>MRGSHHHHHHGSMSNVLIFNVGSSSLTYKVFCSDNIVCSGKSNRVNVTGTEKPFIEHHLNGQIIKIETPILNHPQAAKLIIQFLKENHISIAFVGHRFVHGGSYFKKSAVIDEVVLKELKECLPLAPIHNPSSFGVIEISMKELPTTRQYVAIDTAFHSTISQAERTYAIPQPYQSQYLKFGFHGLSYEYVINSLKN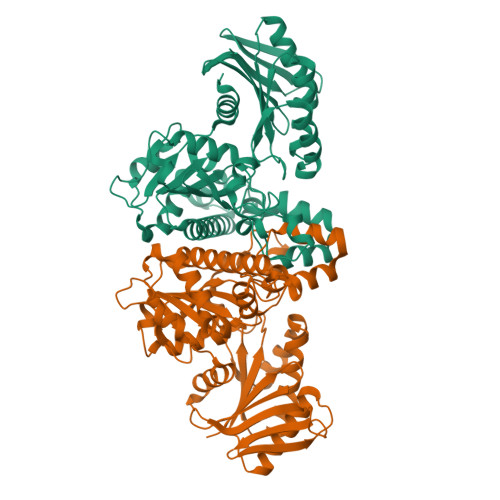VIDVSHSKIIACHLGTGGSSCCGIVNGKSFDTSMGNSTLAGLVMSTRCGDIDPTIPIDMIQQVGIEKVVDILNKKSGLLGVSELSSDMRDILHEIETRGPKAKTCQLAFDVYIKQLAKTIGGLMVEIGGLDLLVFTDQMGLEVWQVRKAICDKMKFLGIELDDSLNEKSMGKKIEFLTMPSSKVQVCVAPNDEELVILQKGKELFQF[2x]> QNGYE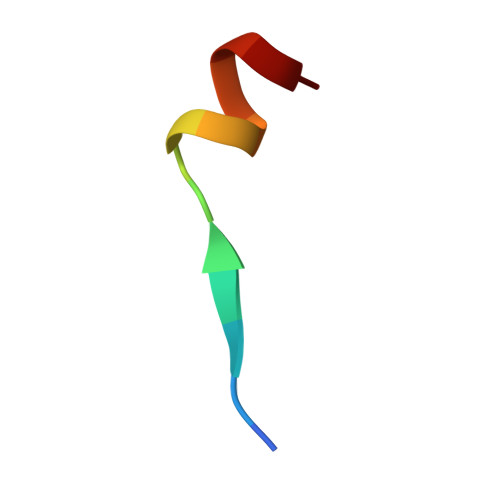NPTYKFFEQ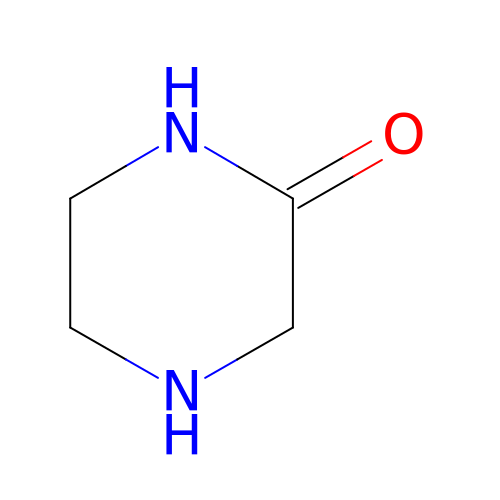piperazin-2-one | C4 H8 N2 O | IWELDVXSEVIIGI-UHFFFAOYSA-N3-[4-(diethylamino)phenoxy]-6-(ethoxycarbonyl)-5,8-dihydroxy-7-oxo-7,8-dihydro-1,8-naphthyridin-1-ium | C21 H23 N3 O6 | 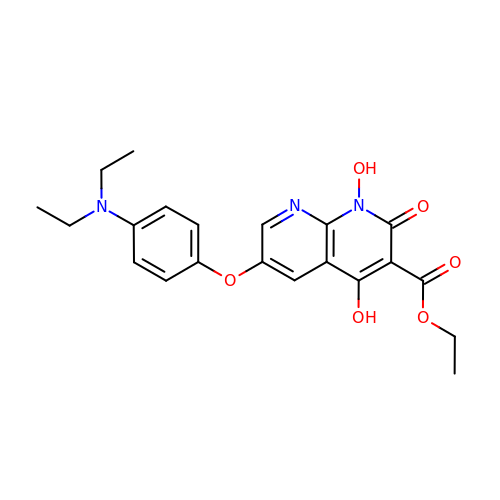ZAOGVQGDYHKJCT-UHFFFAOYSA-N>TRKTYTLTDYLKNTYRLKLYSLRWISDHEYLYKQENNILVFNAEYGNSSVFLENSTFDEFGHSINDYSISPDGQFILLEYNYVKQWRHSYTASYDIYDLNKRQLITEERIPNNTQWVTWSPVGHKLAYVWNNDIYVKIEPNLPSYRITWTGKEDIIYNGITDWVYEEEVFSAYSALWWSPNGTFLAYAQFNDTEVPLIEYSFYSDESLQYPKTVRVPYPKAGAVNPTVKFFVVNTDSLSSVTNATSIQITAPASMLIGDHYLCDVTWATQERISLQWLRRIQNYSVMDICDYDESSGRWNCLVARQHIEMSTTGWVGRFRPSEPHFTLDGNSFYKIISNEEGYRHICYFQIDKKDCTFITKGTWEVIGIEALTSDYLYYISNEYKGMPGGRNLYKIQLSDYTKVTCLSCELNPERCQYYSVSFSKEAKYYQLRCSGPGLPLYTLHSSVNDKGLRVLEDNSALDKMLQNVQMPSKKLDFIILNETKFWYQMILPPHFDKSKKYPLLLDVYAGPCSQKADTVFRLNWATYLASTENIIVASFDGRGSGYQGDKIMHAINRRLGTFEVEDQIEAARQFSKMGFVDNKRIAIWGWSYGGYVTSMVLGSGS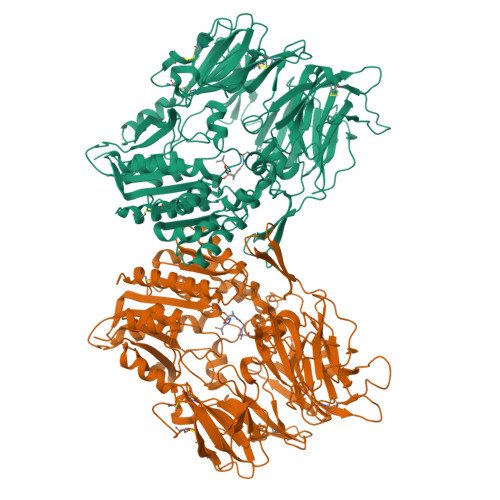GVFKCGIAVAPVSRWEYYDSVYTERYMGLPTPEDNLDHYRNSTVMSRAENFKQVEYLLIHGTADDNVHFQQSAQISKALVDVGVDFQAMWYTDEDHGIASSTAHQHIYTHMSHFIKQCFSLP[4x]Here we showed that the 82-residue hypothetical protein SCO4226 is a nickel binding protein. The overall structure of SCO4226 adopts a ferredoxin-like fold with an α+β structure: five β-strands (β1-5) packing against two α-helices (α1-2). The N-terminal four β-strands β1-4 of one subunit form an antiparallel β-sheet, whereas the C-terminal β5 swaps to the corresponding β-sheet (β1′-4′) of the symmetric subunit, completing an extended antiparallel β-sheet of five strands. Each asymmetric unit contains a dimer of SCO4226, with a buried interface area of about 1100 Å2 on each subunit.

In the structure of Ni-SCO4226, four nickel ions are assigned at the dimer interface, with Ni-1 and Ni-4 on one side, and Ni-2 and Ni-3 on the other. In addition, one citrate molecule is bound to Ni-1 via coordinate bonds. In the dimeric structure of Ni-SCO4226, four nickel ions and one citrate molecule were identified in the electron density map. These four nickel ions are all surface exposed on the dimer interface with varying occupancies from 0.82 to 0.98. Ni-1 and Ni-2 interact with residues within one dimer whereas Ni-3 and Ni-4 are coordinated by residues from two adjacent dimers by symmetric operation. Specifically, Ni-1 is hexa-coordinated by His76-Nδ1, Asp43′-Oδ2, Ser46′-Oγ, and the O4, O7 and O6 atoms of the citrate molecule. Ni-2 is penta-coordinated by His23-Nε2, Ala82′-OXT, and three water molecules. Ni-3 of an octahedral geometry is hexa-coordinated by His3′-Nε2 and Glu38′-Oε2 of one dimer, His12″-Nε2 of the adjacent dimer, and three water molecules (residues from subunit A of the adjacent dimer were labeled with a double prime). Ni-4 coordination is formed by His20′-Nε2 of one dimer, Glu74″-Oε1, Glu74″-Oε2 of the adjacent dimer and three water molecules. The distances for all coordinate bonds are well within the expected range (2.06-2.46 Å). Although the crystal was soaked in a buffer of NiSO4 as high as 0.8 M, the four nickel-binding sites have an occupancy from 0.82 to 0.98.

>[2x]MHHHHHHMAHFMDVHRGMHGITSDQLHQAHQADLAVEKDENVHFEQAWADPASGTIYCLSEGPSAEAVQRVHERAGHKADEIHEVPLSA>[2x]MWKDKEFQVL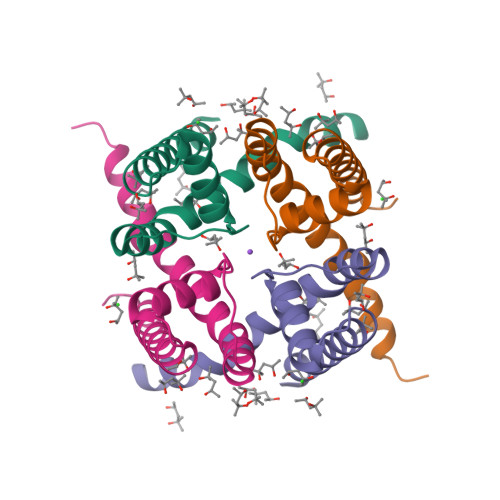FVLTILTLISGTIFYSTVEGLRPIDALYFSVVTLTTVGSDISPQTDFGKIFTILYIFIGIGLVFGFIHKLAVNVQLPSILSNLVPR>[4x]MKDKVYKRPVSILVVIYAQDTKRVLMLQRRDDPDFWQSVTGSVEEGETAPQAAMREVKEEVTI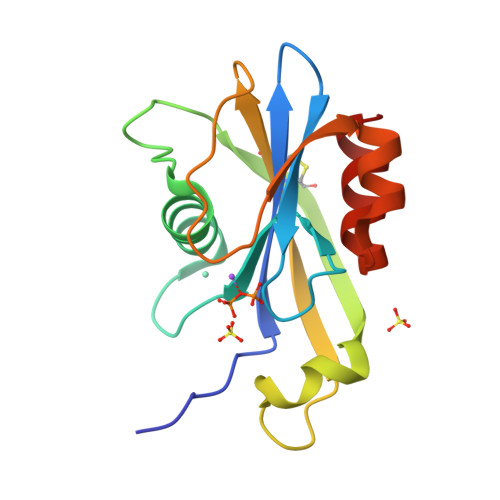DVVAEQLTLIDCQRTVEFEIFSHLRHRYAPGVTRNTESWFCLALPHERQIVFTEHLAYKWLDAPAAAALTKSWSNRQAIEQFVINAA> DEPRTTLDIARIWGLRSTFNWGSGDEHGKELFNTVLDPGLRFYDQDYEGQITPMEYVTGLYNFWSGPIELRFDFVSNAFHTGTVIISAEYNRSSTNTDECQSHSTYTKTFHLGEQKSVHFTVPYIYDTVVRRN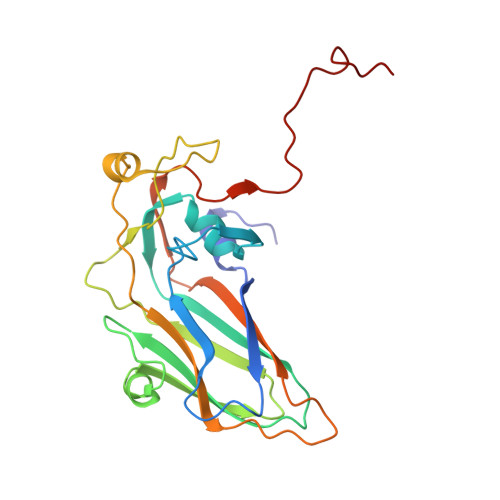TASAYLPVTDYDKVDNVSRAQAMGIRAESKMRVKVRVVNVLRPVASTTSTIEVLVYMRGGKNYALHGLKQSTYWPSNSVVPIDSFPPDGYDP>GSHMGGVEVLDTVPLTEDTQYKVEAVLLPNFGKAATTGNFQSRGLPYTMSDTLGPGAALCYSVAVINLPEIPDAMCEDTMIVWEAYRLETELLFAPQMASSGYQRANGTLAGIEGTQLYFWACGGGPLDVIGINPDPERLKVNEALEGPGNSDVASLQALRKQVNAANFPVELWVADPTKNDNTRYFGRVVGGGVTPPVVSYGNQSTTPLIDENGVGILCTFGSVYLTSADMVGMTGLPGLPTLSADYSNQRTVQAGYGRFFRVHCRQRRIKQ[5x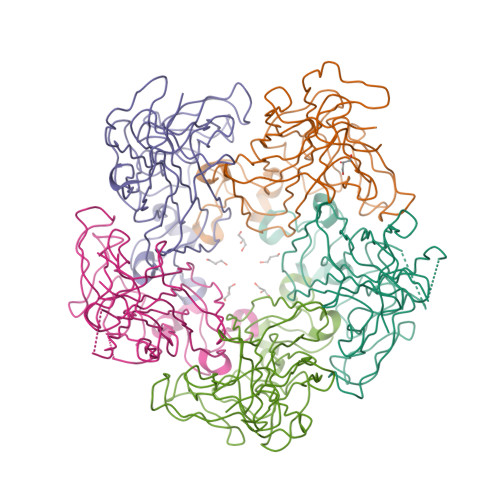]> MAFPAGFGWAAATAAYQVEGGWDADGKGPCVWDTFTHQGGERVFKNQTGDVACGSYTLWEEDLKCIKQLGLTHYRFSLSWSRLLPDGTTGFINQKGIDYYNKIIDDLLKNGVTPIVTLYHFDLPQTLEDQGGWLSEAIIESFDKYAQFCFSTFGDRVKQWITINEANVLSVMSYDLGMFPPGIPHFGTGGYQAAHNLIKAHARSWHSYDSLFRKKQKGMVSLSLFAVWLEPADPNSVSDQEAAKRAITFHLDLFAKPIFIDGDYPEVVKSQIASMSQKQGYPSSRLPEFTEEEKKMIKGTADFFAVQYYTTRLIKYQENKKGELGILQDAEIEFFPDPSWINVDWIYVVPWGVC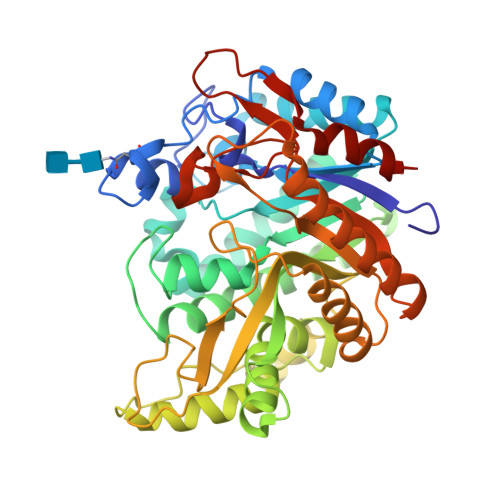KLLKYIKDTYNNPVIYITENGFPQSDPAPLDDTQRWEYFRQTFQELFKAIQLDKVNLQVYCAWSLLDNFEWNQGYSSRFGLFHVDFEDPARPRVPYTSAKEYAKIIRNNGLEAHL Human enteropeptidase (hEP), also known as enterokinase, is an essential enzyme in food digestion and is localized at the brush border of the duodenal and jejunal mucosa. Activated hEP can stimulate the conversion of trypsinogen to trypsin via cleavage of a specific trypsinogen activation peptide, namely Asp-Asp-Asp-Asp-Lys (DDDDK), which is highly conserved in vertebrates. However, the mechanism of hEP activation remains to be established. hEP contains a multi-domain heavy chain and a catalytic light chain, linked by a disulfide bond. The functions of these domains and motifs may be involved in protein anchoring, macromolecular substrate recognition and inhibitor specificity. The light chain is homologous to trypsin-like serine proteinases with a typical Asp-His-Ser (D-H-S) catalytic triad responsible for peptidase activity.

In order to capture the substrate-bound state of hEP, we incubated active hEPwt and hEPmut with the physiological substrate trypsinogen. The association of trypsinogen with active hEPmut was validated by a distinct migration pattern in native gel electrophoresis. Thus, we incubated the active hEPmut with trypsinogen and purified the resulting complex using size exclusion chromatography, and did so in the presence of the cross-linker glutaraldehyde to maintain the complex for cryo-EM analysis. 3D reconstruction of trypsinogen-bound hEPmut yielded a cryo-EM map at a resolution of 4.9 Å, with this relatively low resolution due to the particles having adopted a preferred orientation, resulting in a conformation of active hEPmut with fewer high-resolution features. The overall architecture of the substrate-bound hEPmut was observed to be similar to that of the inactive hEPwt, with extra density observed to be attached to CUB2; this extra density could be attributed to trypsinogen. A full-length model of trypsinogen including its uncleaved N-terminal peptide was constructed based on a prediction using AlphaFold245,46, and this model was docked as a rigid body into the extra density. Note, however, that the N-terminal activation peptide required a minor manual adjustment to be properly fit into the density. This N-terminal tail was inserted into the catalytic pocket, and the cleavage site was located at the center of the active site. Nevertheless, please also note that the resolution of the resolved trypsinogen substrate, including its N-terminal tail, was not sufficient to assign individual amino acid residues. The binding of nafamostat or other covalent inhibitors to the catalytic site apparently results in a change of the conformation of the hEP core region. Substrates such as trypsinogen bind to CUB2 with the N-terminal tail placed into the catalytic site for cleavage.

> ECLPGSSPCTDALTCIKADLFCDGEVNCPDGSDEDNKMCATVCDGRFLLTGSSGSFQATHYPKPSETSVVCQWIIRVNQGLSIKLSFDDFNTYYTDILDIYEGVGSSKILRASIWETNPGTIRIFSNQVTATFLIESDESDYVGFNATYTAFNSSELNNYEKINCNFEDGFCFWVQDLNDDNEWERIQGSTFSPFTGPNFDHTFGNASGFYISTPTGPGGRQERVGLLSLPLDPTLEPACLSFWYHMYGENVHKLSINISNDQNMEKTVFQKEGNYGDNWNYGQVTLNETVKFKVAFNAFKNKILSDIALDDISLTYGICNGSLYPEPTLVPTPPPELPTDCGGPFELWEPNTTFSSTNFPNSYPNLAFCVWILNAQKGKNIQLHFQEFDLENINDVVEIRDGEEADSLLLAVYTGPGPVKDVFSTTNRMTVLLITNDVLARGGFKANFTTGYHLGIPEPCKADHFQCKNGECVPLVNLCDGHLHCEDGSDEADCVRFFNGTTNNNGLVRFRIQSIWHTACAENWTTQISNDVCQLLGLGSGNSSKPIFPTDGGPFVKLNTAPDGHLILTPSQQCLQDSLIRLQCNHKSCGKKLAAQDITPK;> IVGGSNAKEGAWPWVVGLYYGGRLLCGASLVSSDWLVSAAACVYGRNLEPSKWTAILGLHMKSNLTSPQTVPRLIDEIVINPHYNRRRKDNAIAMMHLEFKVNYTDYIQPICLPEENQVFPPGRNCSIAGWGTVVYQGTTANILQEADVPLLSNERCQQQMPEYNITENMICAGYEEGGIDSCQGDAGGPLMCQENNRWFLAGVTSFGYKCALPNRPGVYARVSRFTEWIQSFLH;> APFDDDDKIVGGYNCEENSVPYQVSLNSGYHFCGGSLINEQWVVSAGHCYKSRIQVRLGEHNIEVLEGNEQFINAAKIIRHPQYDRKTLNNDIMLIKLSSRAVINARVSTISLPTAPPATGTKCLISGWGNTASSGADYPDELQCLDAPVLSQAKCEASYPGKITSNMFCVGFLEGGKDSCQGDSGGPVVCNGQLQGVVSWGDGCAQKNKPGVYTKVYNYVKWIKNTIAANS>MKLRASVLIGATILCLILSACSNYAKKVVKQKNHVYTPVYNELIEKYSEIPLNDKLKDTPFMVQVKLPNYKDYLLDNKQVVLTFKLVHHSKKITLIGDANKILQYKNYFQANGARSDIDFYLQPTLNQKGVVMIASNYNDNPNSKEKPQTFDVLQGSQPMLGANTKNLHGYDVSGANNKQVINEVAREKAQLEKINQYYKTLLQDKEQEYTTRKNNQREILETLSNRAGYQMRQNVISSEIFKNGNLNMQAKEEEVREKLQEERENEYLRNQIRSLLSGK[14x]

The H. pylori Cag T4SS is of particular interest because of its role in translocating CagA (a bacterial oncoprotein) into host cells, an important step in gastric cancer pathogenesis. Here we report the use of single particle cryo-EM to determine the structure of a transmembrane Cag T4SS complex extracted and purified from H. pylori. The structure can be divided into three major regions: the OMCC, a periplasmic ring complex (PRC), and a central stalk. The OMCC has a structural organization markedly different from that of T4SS OMCCs in other species, and there is an unexpected symmetry mismatch between the 14-fold-symmetric OMCC and a contiguous 17-fold-symmetric PRC.

Adjacent to CagX, we traced a continuous chain 243 residues long corresponding to CagT. It includes a globular subdomain consisting of two β-sheets followed by a long C-terminal extension of three helices that contribute to the spoke and extend toward the edge of the map. A predicted lipidation site within the N-terminal tail of CagT was not observed in the cryo-EM map, but the N-terminus of CagT is positioned for this interaction with the outer membrane. Consistent with the limited sequence relatedness of CagT to VirB7 homologs, there is relatively little structural relatedness when comparing CagT with VirB7 except for an N-terminal portion that contains little secondary structure. Using symmetry, focused refinement, and symmetry expansion, we determined a 3.7 Å resolution map of the OMCC and a 3.5 Å map of the PRC.>SELAARCLIILFQQLVELARLAIESGDEELLRRVSEWLEEVIKDMRRVVEQALREGNSELAARILIILFQQLVELARLAIESGDEELLRRVSEWLEEVIKDMRRVVEQALREGNSELAARILIILFQQLVELARLAIESGDEELLRRVSEWLEEVIKDMRRVVEQALREGNSELAARILIILFQQLVELARLAIESGDEELLRRVSEWLEEVIKDMRRVVEQALREGNSELAARILIILFQQLVELARLAIESGDEELLRRVSEWLEEVIKDMRRVVEQALREGNSELAARILIILFQQLVELARLAIESGDEELLRRVSEWLEEVIKDMRRVVEQALREGNSELAARILIILFQQLVELARLAIESGDEELLRRVSEWLEEVIKDMRRVVEQALREGNSELACRILIILFQQLVELARLAIESGDEELLRRVSEWLEEVIKDMRRVVEQALREGN[3x]

Circular tandem repeat proteins (‘cTRPs’) are de novo designed protein scaffolds (in this and prior studies, based on antiparallel two-helix bundles) that contain repeated protein sequences and structural motifs and form closed circular structures. While these cTRP constructs have many favorable properties, we have previously noted that their ability to self-assemble from smaller subunits is compromised by relatively limited contacts and small surface areas that are involved in packing between repeats and subunits. Based on those results, we hypothesized that a new generation of computationally designed cTRP proteins with increased repeat size (corresponding to longer secondary structural elements that increase both particle thickness and the number of buried contacts between repeats and protein subunits) would improve both the energetics and the stoichiometric control of self-association. In this study, we describe the de novo design of thick cTRPs (‘tcTRPs’) with repeats composed of longer helical bundles that form a new underlying repeat topology and demonstrate their solution and assembly behaviors, their structural features via X-ray crystallography and CryoEM, and their ability to be functionalized with additional folded protein domains.

Having demonstrated the accuracy and behavior of a designed thick(er) cTRP (tcTRP) harboring nine repeats and a relatively acute radius of curvature between sequential repeats, we next decided to generate and examine a similar tcTRP harboring 24 repeats, corresponding to a considerably larger internal and external diameter and a shallower curvature between consecutive repeats. We therefore attempted to promote the closed toroidal form of this construct by incorporating a pair of cysteine residues at neighboring positions across each subunit interface so that a disulfide staple might lock the protein into the desired closed topology. Based on the tcTRP248 design, an alanine at position 5 and an isoleucine at position 7 (respectively located within the N- and C-terminal repeats of each subunit) were mutated to cysteine residues, with the intention of installing potential disulfide bonds within each interface of the intended tcTRP248 trimeric particle (‘tcTRP248SS’). Reasoning that the designed disulfide bond might only form after cell lysis and exposure to a non-reducing environment (and during that time, would compete with misfolding and fiber formation), we isolated the slowest eluting half of the final peak (corresponding to the expected elution of a correctly formed trimeric particle), concentrated the protein, and subjected it to a second size exclusion step and analysis (‘tcTRP248SS Run #2’). In that second run, the protein now ran as a single uniform peak at a volume and predicted mass corresponding to the desired trimeric assemblage. The structure of the isolated tcTRP248SS construct from the final SEC run was then further examined by CryoEM single particle analysis.> MMQQSRPASDPQVVEAARKEGRLIIYSSTDQSSAQALLDDFRKLYPFIQIEYNDLGTQAIYDRFVSETAAGASSADLLWSSAMELQVKLASEGYALPYDSPEAKNWPANARLGNLAYSTTLEPAVVVYNKRFLKPEEVPTTREGLARLLQEPRMRGRVATWDPERSAVGFTILKADYDRFPAFQELARAFGKAQAALYSSTGAAFEKVISGEHYLAYGFFGSFALLRQRTVKDLGIAYLTDGTVAIQRVAFINKRAAHPNAAKLFLD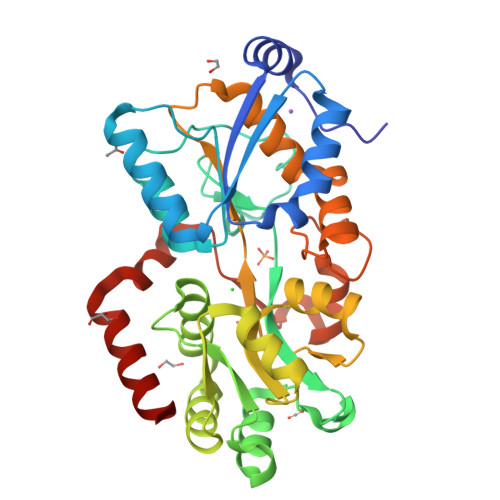YLLSLRGQNLMAYTALIFARRETVVGEATPQALYKAVGGKDKVYAIPVSTEILKNLDPAERMRFLTFWRQAVRGQ(4-ETHYLPHENYL)SULFAMIC ACID | C8 H11 N O3 S | 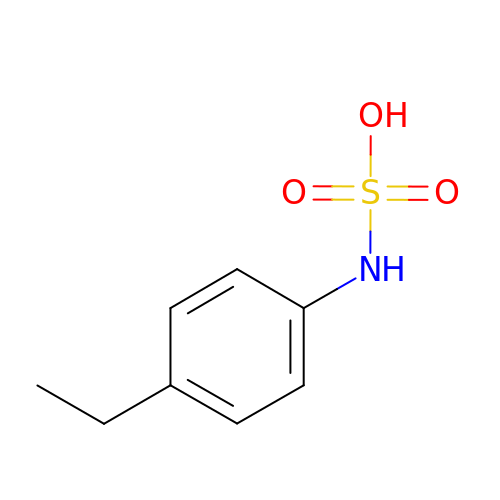HXARYYGNSVTEFC-UHFFFAOYSA-N>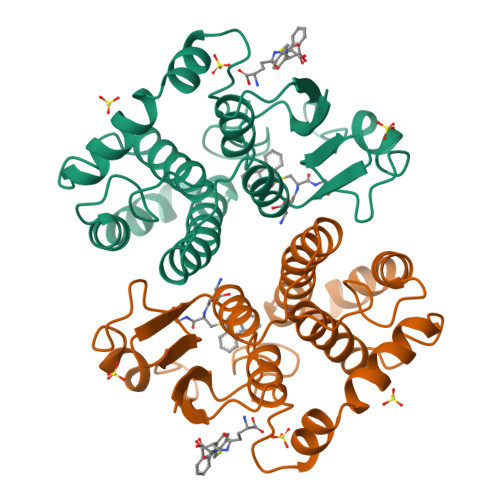 PMILGYWNVRGLTHPIRLLLEYTDSSYEEKRYAMGDAPDYDRSQWLNEKFKLGLDFPNLPYLIDGSRKITQSNAIMRYLARKHHLCGETEEERIRVDVLENQAMDTRLQLAMVCYSPDFERKKPEYLEGLPEKMKLYSEFLGKQPWFAGNKITYVDFLVYDVLDQHRIFEPKCLDAFPNLKDFVARFEGLKKISDYMKSGRFLSKPIFAKMAFWNPK>SNAMVDKRESYTKEDLEASGRGELFGAGGPPLPAGNMLMMDRIVKMIEDGGSHNKGYVEAELDINPDLWFFGCHFIGDPVMPGCLGLDAMWQLVGFYLGWLGGEGKGRALGVGEVKFTGQVLPDAKKVTYRINFKRVIMRKLIMGVADGEVLVDGKVIYTATDLKV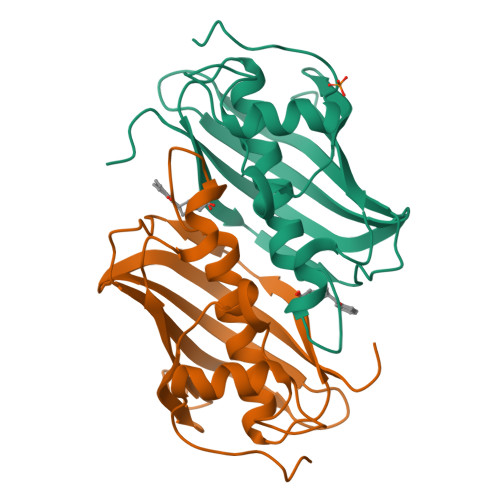GLFKDTNAF[2x]>[3x]MAKFFIDRPIFAWVISIFIIAAGIFGIKSLPVSQYPSVAAPTITLHAIYPGASAQVMEGSVLSVIERNMNGVEGLDYMSTSADSSGSGSVSLTFTPDTDENLAQVEVQNKLSEVLSTLPATVQQYGVTVSKARSNFLMIVMLSSDVQSTEEMNDYAQRNVVPELQRIEGVGQVRLFGAQRAMRIWVDPKKLQNYNLSFADVGSALSAQNIQISAGSIGSLPAVRGQTVTATVTAQGQLGTAEEFGNVILRANTDGSNIYLKDVAKVGLGMEDYSSSTRLNGVNTTGMAVMLSNSGNAMATAKAVKERLAVLEKYFPQGMSWKT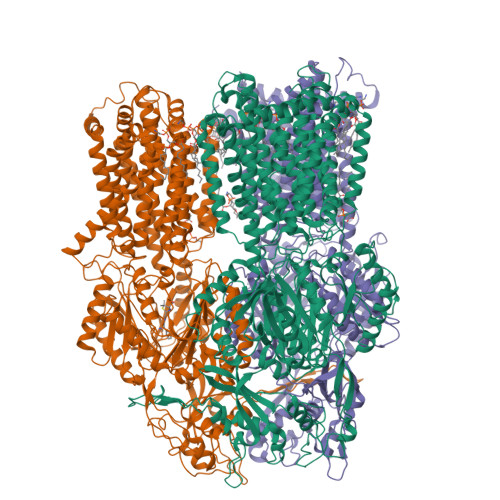PYDTSKFVEISIEKVIHTLIEAMVLVFVVMYLFLQNIRYTLIPTIVVPISLLGGFAFISYMGMSINVLTMFAMILVIGIVVDDAIVVVENVERIMAGEGLPPKEATKKAMGQISGAVIGITAVLISVFVPLAMFSGAAGNIYKQFALTMASSIAFSAFLALTLTPALCATMLKTIPKGHHEEKKGFFGWFNKKFDSWTHGYEGRVAKVLRKTFRMMVVYIGLAVVGVFLFMRLPTSFLPTEDQGFVMVSVQLPAGATKERTDATLAQVTQLAKSIPEIENIITVSGFSFSGSGQNMAMGFAILKDWNERTASGSDAVAVAGKLTGMMMGTLKDGFGIAVVPPPILELGNGSGLSINLQDRNNTGHTALLAKRNELIQKMRASGLFDPSTVRAGGLEDSPQLKIDINRAAAAAQGVSFADIRTALASALSSSYVSDFPNQGRLQRVMVQADGDARMQPADILNLTVPNSSGIAVPLSSIATVSWQMGTEQSVRFNGYPAMELSGSPATGVSTGQAMEAVQKMVDELGSGYSLEWGGQSREEAKGGSQTIALYALAAVAVFLVLAALYESWSIPLAVLLVMPLGLAGAAAGVTGRNLFEGLLGSVPSFANDIYFQVGFVTVMGLSAKNAILIIEFAKDLQAQGKSAVEAALEAARLRFRPIIMTSFAFILGVVPLYIAGGASSASQRAIGTTVFWGMLIGTLLSVFLVPLFYVVVRKFFKETAHEHEM> KH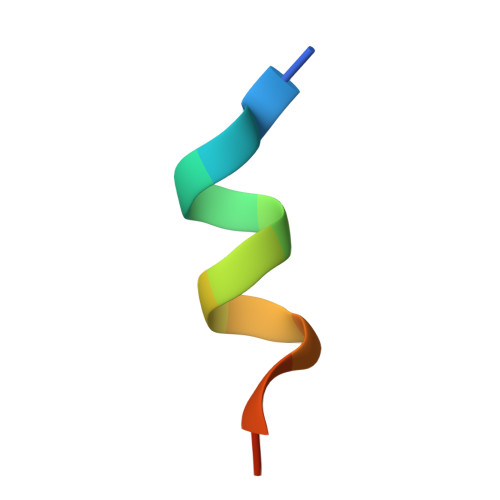KILHRLLQDSSY> AVPFVEDWDLVQTLGEGAYGEVQLAVNRVTEEAVAVKIVDMKRAVDCPENIKKEICINKMLNHENVVKFYGHRREGNI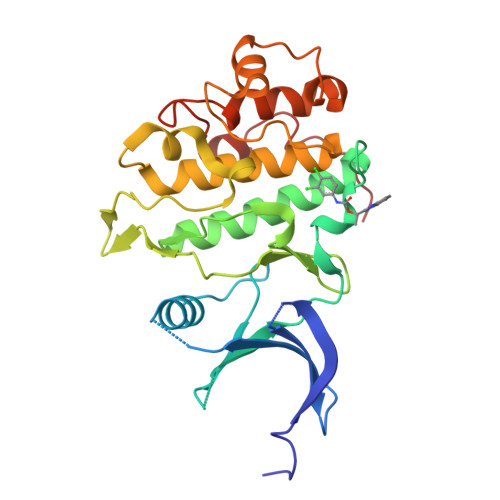QYLFLEYCSGGELFDRIEPDIGMPEPDAQRFFHQLMAGVVYLHGIGITHRDIKPENLLLDERDNLKISDFGLATVFRYNNRERLLNKMCGTLPYVAPELLKRREFHAEPVDVWSCGIVLTAMLAGELPWDQPSDSCQEYSDWKEKKTYLNPWKKIDSAPLALLHKILVENPSARITIPDIKKDRWYNKPLKKG>[3x]MTYETILVERDQRVGIIT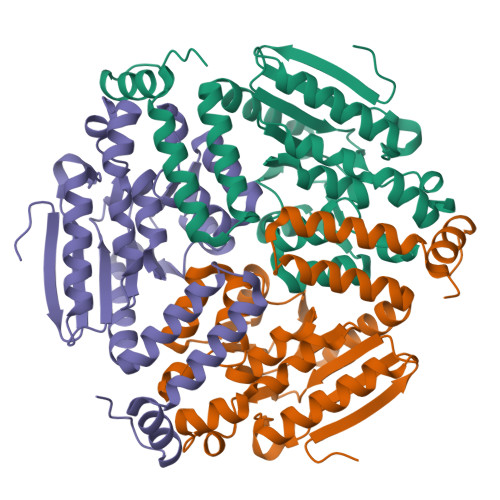LNRPQALNALNSQVMNEVTSAATELDDDPDIGAIIITGSAKAFAAGADIKEMADLTFADAFTADFFATWGKLAAVRTPTIAAVAGYALGGGCELAMMCDVLIAADTAKFGQPQIKLGVLPGMGGSQRLTRAIGKAKAMDLILTGRTMDAAEAERSGLVSRVVPADDLLTEARATATTISQMSASAARMAKEAVNRAFESSLSEGLLYERRLFHSAFATEDQSEGMAAFIEKRAPQFTHR> EDMPVERILEAELAVEPKTETYVEANMGLNPSSPNDPVTNICQAADKQLFTLVEWAKRIPHFSELPLDDQVILLRAGWNELLIASFSHRSIAVKDGILLATGLHVHRNSAHSAGVGAIFDRVLTELVSKMRDMQMDKTELGCLRAIVLFNPDSKGLSNPAEVEALREKVYASLEAYCKHKYPEQPGRFAKLLLRLPALRSIGLKCLEHLFFFKLIGDTPIDTFLM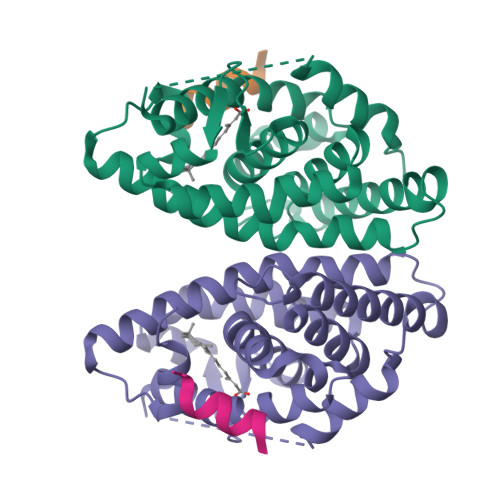EMLEAP;> KHKILHRLLQD>[2x]GPLGSSTQSHMFDGISLTEHQRQQMRDLMQQARHEQPPVNVSE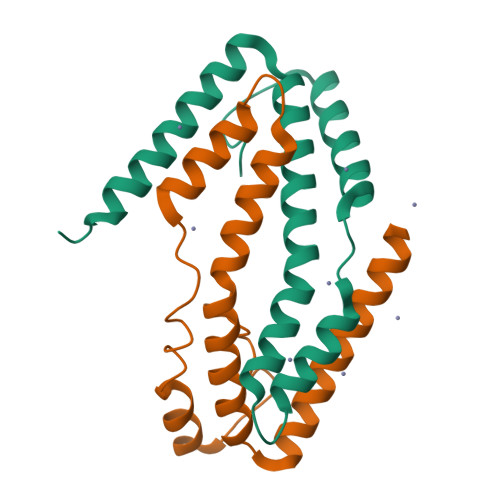LETMHRLVTAENFDENAVRAQAEKMANEQIARQVEMAKVRNQMYRLLTPEQQAVLNEKHQQRMEQLRDVTQWQK> MRTLKVQALWDGEAGVWVAES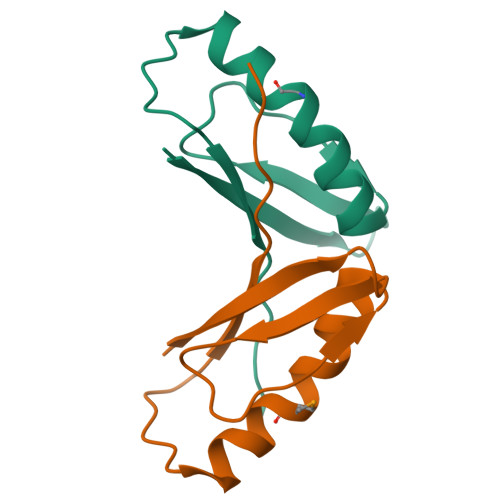DDVPGLATEAATLEELLAKLAVMVPELLEENGVALELPVELRLEATRPLVFS>[2x]QGMIMTSDIKLLDYLRVRRSTPALQLSEPGPSKGEIEEILRLAVRVPDHGKLAPWRFVVYRGEERVRLS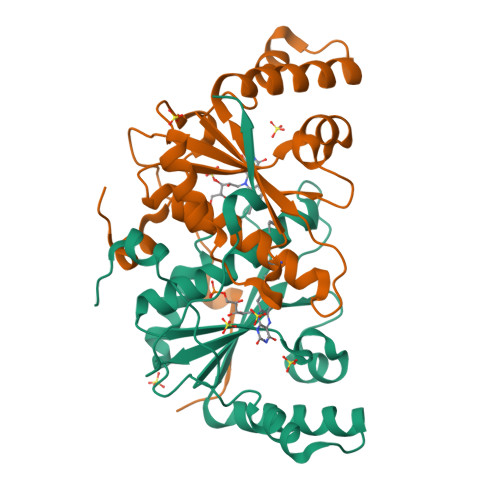EAALRIALEKNPDLDLQQQEAERTRFTRAPVVIAVISTAKPHFKIPEWEQVMSAGAVCLNVIFAANASGFAANWLTEWLAFDPAFLAEIGVSAEEKVAGYIHIGSTTFPPVERPRPELADVVTWVGDV> GDPVEDIIHDALSSTVRRAITSGQDVNTAAGTAPSSHRLETGRVPALQAAETGATSNATDENMIETRCVMNRNGVLEATISHFFSRSGLVGVVNLTDGGTDTTGYAVWDIDIMGFVQLRRKCEMFTYMRFNAEFTFVTTTENGEARPFMLQYMYVPPGAPKPTGRDAFQWQTATNPSVFVKLTDPPAQVSVPFMSPASAYQWFYDGYPTFGQHPETSNTTYGQCPNNMMGTFAVRVVSRVASQLKLQTRVYMKLKHVRAWIPRPIRSQPYLLKNFPNYDSSKITYSARDRASIKQANM;> SPSVEACGYSDRVAQLTVGNSSITTQEAANIVLAYGEWPEYCPDTDATAVDKPTRPDVSVNRFYTLDSKMWQENSTGWYWKFPDVLNKTGVFGQNAQFHYLYRSGFCLHVQCNASKFHQGALLVAVIPEFVLAGRGSNTKPNEAPHPGFNTTFPGTAGASFNDPYVLDSGVPLSQSL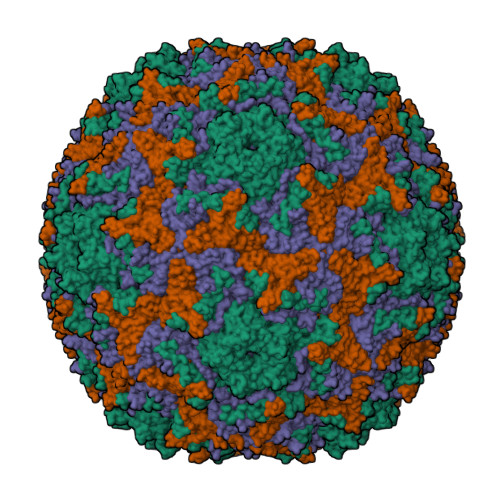IYPHQWINLRTNNCATIIVPYINAVPFDSAINHSNFGLIVVPVSPLKYSSGATTAIPITVTIAPLNSEFGGLRQAVSQ;> GLPTELRPGTNQFLTTEDDTAAPILPGFSPTPSIHIPGEVRSLLELCRVETILEVNNTTDATGLNRLLIPVSAQNKADELCAAFMVDPGRIGPWQSTLVGQICRYYTQWSGSLKVTFMFTGSFMATGKMLIAYSPPGSAQPANRETAMLGTHVIWDFGLQSSVSLVIPWISNTHFRTAKTGGNYDYYTAGVVTLWYQTNYVVPPETPGEAYIIAMGAAQDNFTLKICKDTDEVTQQAVLQ;> MGAQVSSQRSGSHETGNVATGGSTINFTNINYYKDSYAASASRQDFTQDPKKFTQPVLDSIRELSAPLN> AMADIGSYKL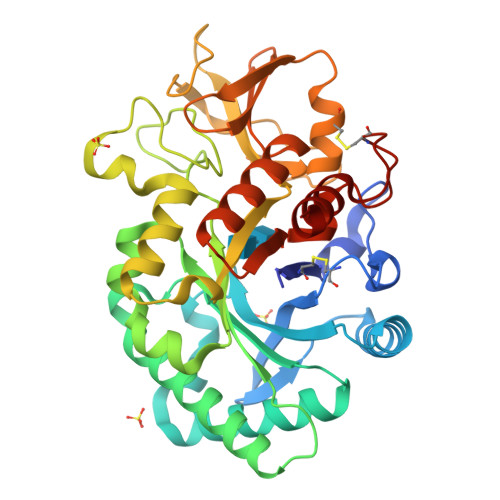VCYFTNWSQDRQEPGKFTPENIDPFLCSHLIYSFASIENNKVIIKDKSEVMLYQTINSLKTKNPKLKILLSIGGYLFGSKGFHPMVDSSTSRLEFINSIILFLRNHNFDGLDVSWIYPDQKENTHFTVLIHELAEAFQKDFTKSTKERLLLTVGVSAGRQMIDNSYQVEKLAKDLDFINLLSFDFHGSWEKPLITGHNSPLSKGWQDRGPSSYYNVEYAVGYWIHKGMPSEKVVMGIPTYGHSFTLASAETTVGAPASGPGAAGPITESSGFLAYYEICQFLKGAKITWLQDQQVPYAVKGNQWVGYDDVKSMETKVQFLKNLNLGGAMIWSIDMDDFTGKSCNQGPYPLVQAVKRSLGSL2-acetamido-2-deoxy-6-O-sulfo-alpha-D-glucopyranose | C8 H15 N O9 S | 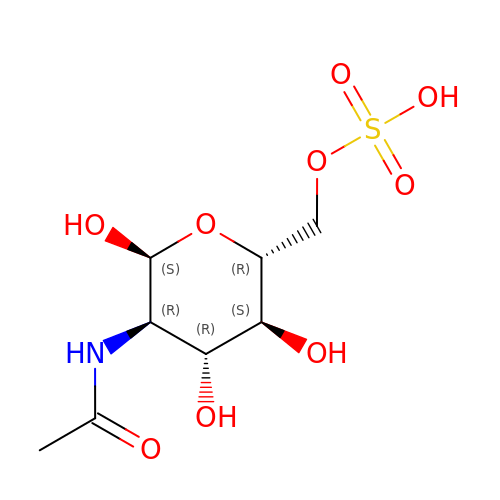WJFVEEAIYIOATH-PVFLNQBWSA-N3-methyl-4-({3-[3-methyl-5-(trifluoromethyl)phenyl]-1H-pyrazol-5-yl}carbamoyl)benzoic acid | C20 H16 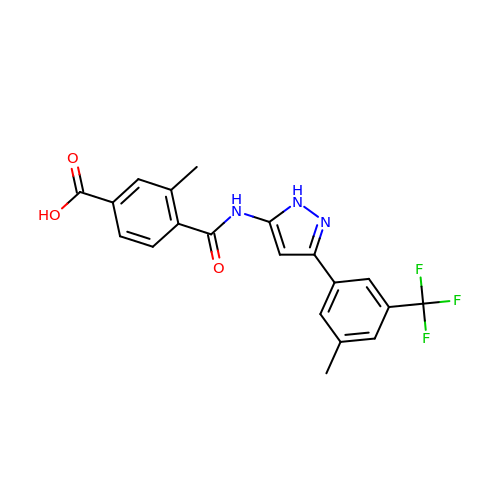F3 N3 O3 | MLGFDWKUOYDRDY-UHFFFAOYSA-N> VQVLITDSGQRTGTGSALMAMKDAGVNTYRWQGGEQRPATIISEPDRNVRYARLAGDFAASVKAGEESVAQVSGVREQAILTQAIRSELKTQGVLGHPEVTMTALSPVWLDSRSRYLRDMYRPGMVMEQWNPETRSHDRYVIDRVTAQSHSLTLRDAQGETQVVRISSLDSSWSLFRPEKMPVADGERLRVTGKIPGLRVSGGDRLQVASVSEDAMTVVVPGRAEPASLPVSDSPFTALKLENGWVETPGHSVSDSATVFASVTQMAMDNATLNGLARSGRDVRLYS

In the paradigm F and related R1 plasmid systems the 192 kDA protein TraI is the substrate of the T4SS encoded by the tra genes (Everett and Willetts, 1980; Reygers et al., 1991; Lang et al., 2010; Dostal et al., 2011). This bifunctional protein includes both the relaxase activity and a helicase that assists unwinding of the T-strand. A second group, which includes TraI, have larger, internally positioned signals. These regions of TraI, called translocation signals (TS) A (530–816) and B (1255–1564), target the relaxosome to the secretion machinery (Lang et al., 2010). In this study we report the crystal structure of the TSA domain of the TraI protein from the R1 plasmid.

Analysis of the protein crystals on an SDS-PAGE indicated that, in fact, an even smaller fragment had crystallized, TSAcryst: N-terminal sequencing of the crystallized fragment showed the fragment to start at residue 570. No attempt was made to characterize the C-terminal sequence of the crystallized fragment. This fragment of TSA crystallized in the space group P41212 with one molecule in the asymmetric unit. The structure was solved using the single wavelength anomalous dispersion phasing method (Rice et al., 2000) from a SelenoMethionine (SeMet)-substituted variant of TSA (TSA contains six methionines), and refined to a final resolution of 1.85 Å. A model was built between residues 575 and 786. The crystal structure of the TSA domain of the R1 plasmid is composed of three structural domains named ‘2A, 2B and 2B-like’ for reasons that are explained below. Domain 2B is made of sequences inserted within domain 2A, while domain 2B-like is made of sequences inserted within domain 2B. A structural homology search using the DALI server was performed which resulted in the identification of domain 2 of SF1B helicases as TSA's closest structural homologue: the RecD subunit of the RecBCD helicase ranked first with a Z-score of 8.9 (a highly significant score), followed by other SF1B helicase structures. Thus, due to the high structural homology between TSA and SF1B helicase subdomains, we can conclude that TSA is part of a helicase structure, its two first domains, 2A and 2B matching parts of the structure of the 2A and 2B domains of SF1B helicases. Thus the 2B-like domain of TraI constitutes a previously uncharacterized addition to the helicase fold, which here serves as a signal recognition surface linked to substrate transport. Five mutations resulted in significant loss of translocation activity: A593V, D714N, Q736N, S739A and S739N, indicating that four residues, 593, 714, 736 and 739 play an important role as recognition surfaces for substrate export.>SNAMSEEKSEEVQETRPTPRLNERILSSLSRRSVAAHPWHDLEIGPGAPNIFNCVVEITKGSKVKYELDKKTGMIKVDRILYSSVVYPHNYGFIPRTLCEDNDPLDVLVLMQEPVLPGCFLRARAIGLMPMIDQGEKDDKIIAVCADDPEYKHYTDFKELQPHRLMEIKRFFEDYKKNEN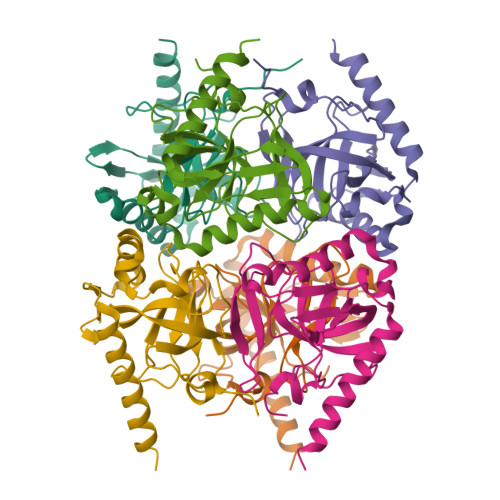KEVAVNEFLPPSTAVEAIQHSMDLYAEYILHTLR[4x]>[11x]TGTANTLFGT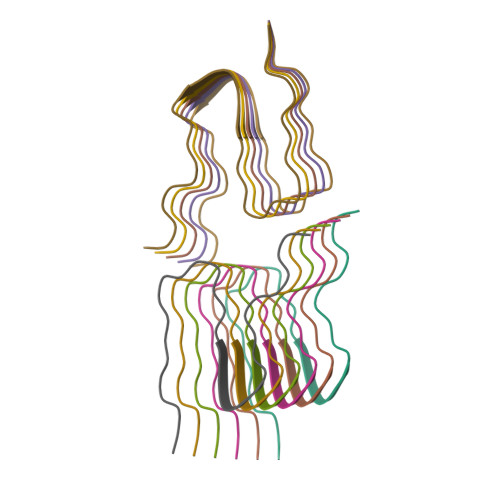ASTGTSLFSSQNNAFAQNKPTGFGNFGTST PYRIDINE-2,6-DICARBOXYLIC ACID | C7 H5 N O4 | 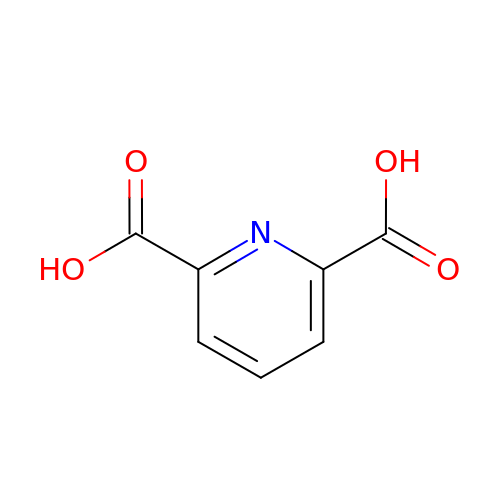WJJMNDUMQPNECX-UHFFFAOYSA-N> MADKRAHHNALERKRRDHIKDSFHSLRDSVPSLQGEKASRAQILDKATEYIQYMRRKNHTHQQDIDD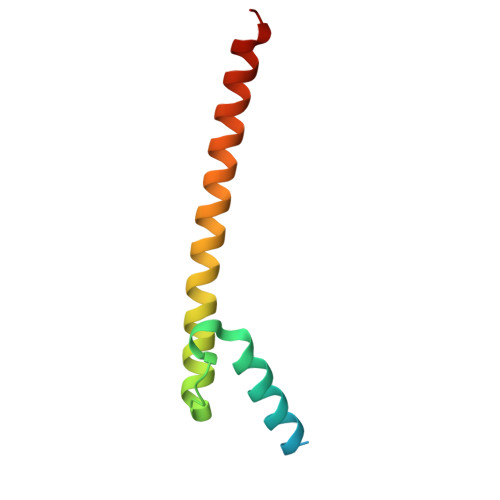LKRQNALLEQQVRALE Clinical Tv isolates are frequently found infected with one or more strain of the double-stranded RNA (dsRNA) Trichomonas vaginalis viruses (TVVs), belonging to the Trichomonasvirus genus within totiviruses. Here, we have determined the structure of TVV2 by cryo-electron microscopy (cryoEM) at 3.6 Å resolution and derived an atomic model of its capsid. TVV2 has an icosahedral, T = 2*, capsid comprised of 60 copies of the icosahedral asymmetric unit (a dimer of the two capsid shell protein [CSP] conformers, CSP-A and CSP-B), typical of icosahedral dsRNA virus capsids. Among totiviruses, the single capsid layer is responsible for protecting and sequestering the viral genome while facilitating RdRp activity and the egression of viral mRNA into the cytosol.

Subparticle reconstruction about the I5 vertices improved the resolution of the decameric complex to ∼3.6 Å by the same FSC criteria. Using the molecular modeling software Coot, and guided by secondary structural element predictions from Phyre2 (33), TVV2 CSP residues 37 to 700 were built into a single decamer subunit, denoted capsid shell protein conformer A (CSP-A), nearest the I5 vertex. CSP-A was used as a homology model for building residues 37 to 701 into the alternative subunit (CSP-B) situated further from the I5 vertices. This A-B pair constitutes the principle icosahedral asymmetric unit (IAU) of the viral capsid, and model quality can be observed based on fit in the cryoEM map. Analysis by the Dali server indicated a root mean square deviation (rmsd) of 1.4 Å calculated between all 664 aligned Cα atoms (Z-score = 47.7) of the pair. Notably, we observe an unwinding of α4 and α15 from CSP-A to CSP-B to accommodate the interface with the adjacent CSP-A subunits. As noted in the planar view, channels spanning the width of the capsid shell are located at the I5 vertices. These I5 channels are lined with residues extending from loops between α3 to α4 and β7 to β8 within the apical domain. Closer inspection of the decamer model from the outside reveals the residues lysine 157, arginine 159, and asparagine 255 from all 5 CSP-As lining this channel. The channel measures approximately 9.2 Å in diameter nearest the capsid interior, to 12.8 Å near the exterior, and this contrasts with the 16 to 20 Å I5 channel of TVV1 derived from a lower-resolution cryoEM map in a previous investigation. In the TVV2 CSP-A we observe positively charged residues (R74, K523, R525, K539, R646, and R653) arranged on the cleft exterior generating a positively charged region similar to that observed in ScV-L-A.

>[2x]SNPRLTKVLDEMSKKPCVNINEIRKMIRNFQPQFIQPRNGNRPNAQPRTVDSFEWVVRIQSTVETQLLGATNTVPQQTLNLDISFTDDSTTITPASIPGSISMLDNSRHIPAIQSMIQNFKARYLGSLQDTAQLQSPQYPQLLAYLFGQLIAIKDRLDLFRPSNPLSLADALFGFTLAQNARPRYDDHRHAKACQGPLVIPAATNSDCGPCGFVQINANQGLTLPLGACLFVNPETVNDQSFQDFLWLIFATHHRMPNQMQNNWPFSLNIVSTCAAPGRQAPHAGELTDERVRLALDTGHRILLSMFNDDEETLRYYQRKGIETMFRPCCFYTEGGLLRKATRYVSMVPLNGLYYYNGATSYVVSPIHTDAHPGITAAIESFVDIMVLQAVFSFSGPKVVAAKVNASQIDAAMVFGPAVAEGDGFVYDPLRPAPPLSAFYTEFIHRPAEQRIFQMAMSQIYGSHAPLIIANVINSIHNCKTKIVNNKLRATFVRRPPGAPHLKADTAIINRFHDPELAYALGILADGIAPLDGSHEYNVLDELDYLFNGGDIRNCFGLNALNTRGLGQIVHIRPKREPGKRPRRGFYTTLDGQVHPVTQDAPLDEIYHWRDHGNLTRPYSCHILDSQGLEFADVSNGRSRGKILVVVNSPLKTCAAYQGPSFAPK> ECHLSDLLQQLTSVNASKPSERGLVRQEEAEDPACIPIFWVSKWVDYSDKYGLGYQLCDNSVGVLFN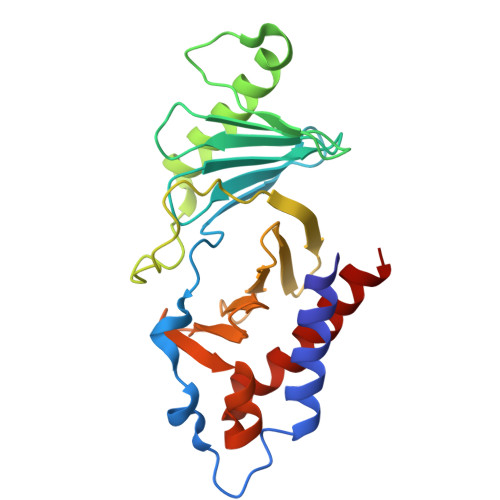DSTRLILYNDGDSLQYIERDGTESYLTVSSHPNSLMKKITLLNYFRNYMSEHLLKAGANITPREGDELARLPYLRTWFRTRSAIILHLSNGTVQINFFQDHTKLILCPLMAAVTYINEKRDFQTYRLSLLEEYGCCKELASRLRYARTMVDKLLSSR>MDDAVARAVEIVRKQGVADANLVRMGDKSIMFSEKGDAFIMYGKQGRSWIALFDPVGPRQALPDLIWRFVETARAAGCRSVFYQISPALLSYCADAGLRAFKLGELAVVNLANFELKGGKWANLRQTASRAVRDGLEFAVIEPQDIPDVLDQLAHVSDTWLADHNAKEKSFSLGAFDPDYVCSQPVGVLKKDGKIVAFANILMTETKEEGSVDLMRFSPDAPKGSMDFLFVQILEYLKGEGFQRFNLGMAPLSGMSRRESAPVWDRVGGTVFEHGERFYNFKGLRAFKSKFHPEWQPRYLAVSGGVSPMIALMDATFLIGGGKLAAALEHHHHHH[2x]

As a large family of membrane proteins crucial for bacterial physiology and virulence, the Multiple Peptide Resistance Factors (MprFs) utilize two separate domains to synthesize and translocate aminoacyl phospholipids to the outer leaflets of bacterial membranes. The function of MprFs enables Staphylococcus aureus and other pathogenic bacteria to acquire resistance to daptomycin and cationic antimicrobial peptides. Here we present cryo-electron microscopy structures of MprF homodimer from Rhizobium tropici (RtMprF) at two different states in complex with lysyl-phosphatidylglycerol (LysPG). RtMprF contains a membrane-embedded lipid-flippase domain with two deep cavities opening toward the inner and outer leaflets of the membrane respectively.

The crystal structure of the catalytic domain of RtMprF in the C-terminal region has been solved at 2.0 Å resolution, and serves as the initial model for building the corresponding region in the cryo-EM structures of the full-length RtMprF. The synthase domain of RtMprF (Pro539-Gly860) superposes well with those of PaMprF and BlMprF (root-mean-square deviation of α-carbons at 0.977 and 1.297 Å, respectively). They share similar tandem repeats of the General Control Nonderepressible 5 (a histone acetyltransferase of a transcriptional regulatory complex) related N-acetyltransferase (GNAT) folds (GNAT folds 1 and 2). The potential binding site of lysyl-tRNA in the synthase domain of RtMprF is located at the cleft between GNAT folds 1 and 2, according to the previous studies on an alanyl transferase FemX involved in peptidoglycan biosynthesis (in complex with an aminoacyl-tRNA analog) and BlMprF in complex with L-lysine amide (LYN).methyl 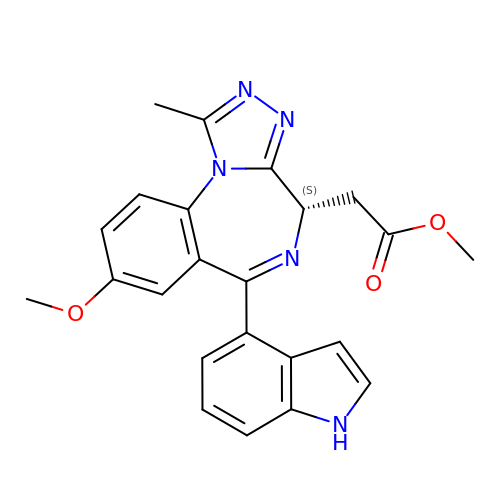[(4S)-6-(1H-indol-4-yl)-8-methoxy-1-methyl-4H-[1,2,4]triazolo[4,3-a][1,4]benzodiazepin-4-yl]acetate | C23 H21 N5 O3 | RARZHTSXOQRRPR-IBGZPJMESA-N> SMLKREDWYDLTRTTNWTPKYVTENELFPEEMSGARGISMEAWEKYDEPYKITYPEYVSIQREKDSGAYSIKAALERDGFVDRADPGWVSTMQLHFGAIALEEYAASTAEARMARFAKAPGNRNMATFGMMDENRHGQIQLYFPYANVKR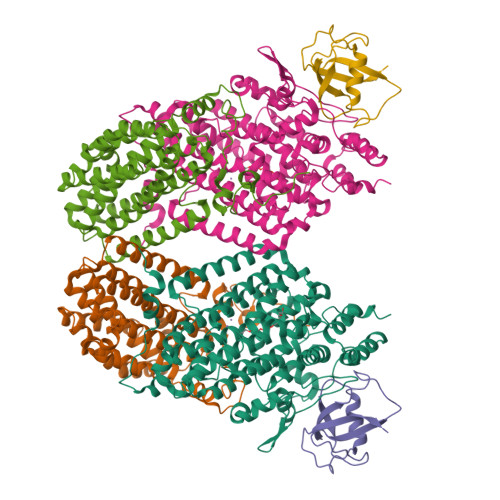SRKWDWAHKAIHTNEWAAIAARSFFDDMMMTRDSVAVSIMLTFAFETGFTNMQFLGLAADAAEAGDHTFASLISSIQTDESRHAQQGGPSLKILVENGKKDEAQQMVDVAIWRSWKLFSVLTGPIMDYYTPLESRNQSFKEFMLEWIVAQFERQLLDLGLDKPWYWDQFMQDLDETHHGMHLGVWYWRPTVWWDPAAGVSPEEREWLEEKYPGWNDTWGQCWDVITDNLVNGKPELTVPETLPTICNMCNLPIAHTPGNKWNVKDYQLEYEGRLYHFGSEADRWCFQIDPERYKNHTNLVDRFLKGEIQPADLAGALMYMSLEPGVMGDDAHDYEWVKAYQ;> ALKPLKTWSHLAGNRRRPSEYEVVSTNLHYFTDNPERPWELDSNLPMQTWYKKYCFDSPLKHDDWNAFRDPDQLVYRTYNLLQDGQESYVQGLFDQLNDRGHDQMLTREWVETLARFYTPARYLFHALQMGSVYIHQIAPASTITNCATYETADHLRWLTHTAYRTRELANCYPDVGFGKRERDVWENDPAWQGFRELIEKALIAWDWGEAFTAINLVTKPAVEEALLQQLGSLAQSEGDTLLGLLAQAQKRDAERHRRWSSALVKMALEKEGNREVLQKWVAKWEPLADKAIEAYCSALPDGENAIVEAKSASRYVRQMMGL;> TFPIMSNFERDFVIQLVPVDTEDTMDQVAEKCAYHSINRRVHPQPEKILRVRRHEDGTLFPRGMIVSDAGLRPTETLDIIFMD> GAMATLYKKAGLLVTIPLIKGPKGFGFAIADSPTGQKVKMILDSQWCQGLQKGDIIKEIYHQNVQNLTHLQVVEVLKQFPVGADVPLLIL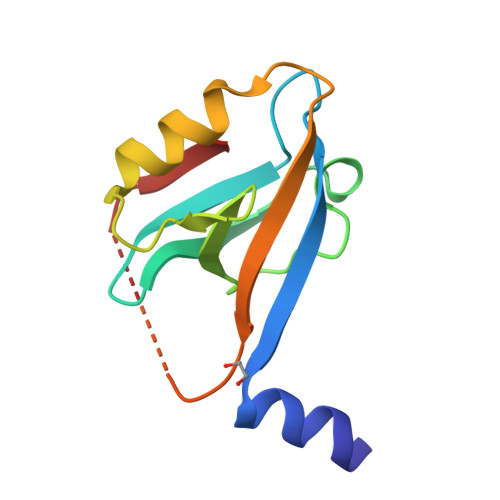RGGPPSPTKTAKMGSGSGQITKV>MGKNLQALAQLYKNALLNDVLPFWENHSLDSEGGYFTCLDRQGKVYDTDKFIWLQNRQVWTFSMLCNQLEKRENWLKIARNGAKFLAQHGRDDEGNWYFALTRGGEPLVQPYNIFSDCFAAMAFSQYALASGEEWAKDVAMQAYNNVLRRKDNPKGKYTKTYPGTRPMKALAVPMILANLTLEMEWLLPQETLENVLAATVQEVMGDFLDQEQGLMYENVAPDGSHIDCFEGRLINPGHGIEAMWFIMDIARRKNDSKTINQAVDVVLNILNFAWDNEYGGLYYFMDAAGHPPQQLEWDQKLWWVHLESLVALAMGYRLTGRDACWAWYQKMHDYSWQHFADPEYGEWFGYLNRRGEVLLN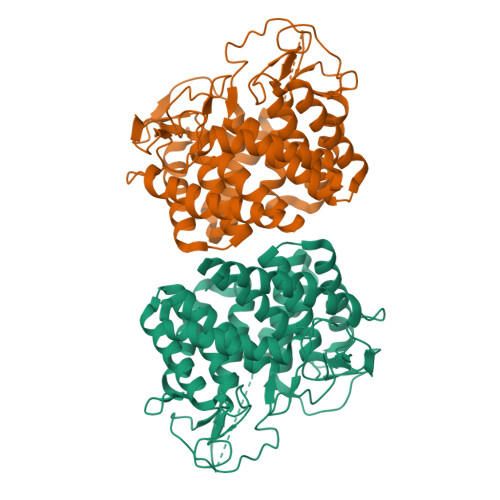LKGGKWKGCFHVPRAMYLCWQQFEALS[2x]> SMKLDIKKTFSNRSDRVKGIDFHPTEPWVLTTLYSGRVEIWNYETQVEVRSIQVTETPVRAGKFIARKNWIIVGSDDFRIRVFNYNTGEKVVDFEAHPDYIRSIAVHPTKPYVLSGSDDLTVKLWNWENNWALEQTFEGHEHFVMCVAFNPKDPSTFASGCLDRTVKVWSLGQSTPNFTLTTGQERGVNYVDYYPLPDKPYMITASDDLTIKIWDYQTKSCVATLEGHMSNVSFAVFHPTLPIIISGSEDGTLKIWNSSTYKVEKTLNVGLERSWCIATHPTGRKNYIASGFDNGFTVLSLG;> GVKLHYT

Hence, this loss of critical proteins has the potential to compromise ER proteostasis and generate cellular stress. This challenge to normal metabolism is overcome by the activity of the cytosolic coatomer protein I (COPI) polymer, whose repeating unit is the coatomer, a 560 kDa complex of seven distinct gene products (α-, β-, β′-, γ-, δ-, ε-, and ζ-COPI)25–31. Overall, the coatomer functions to retrieve the escaped “client” proteins, such as type I membrane proteins, from cis-Golgi back to ER by retrograde trafficking. In particular, the S protein – a type I membrane protein – is delivered to the ERGIC from both the ER (by anterograde trafficking) and the Golgi (by retrograde trafficking)3,10–12. Here we utilize recombinant SARS-CoV-2 S proteins and tail peptides, including constructs with enhanced mimicry of the coatomer binding motif (clientized S protein), to elucidate the atomic structure of the S-coatomer interface.

To determine an atomic-level understanding of S-coatomer interactions, we attempted co-crystallization of αWD40 with either wild-type (1267Gly-Val-Lys-Leu-His-Tyr-Thr1273) or clientized (1267Gly-Val-Lys-Leu-His-Tyr-Glu1273) S tail heptapeptides. However, in our co-crystallization experiments, contacts between symmetry-related αWD40 molecules occluded the binding site and no S tail peptide density was observed. Hence, we subsequently adopted a previously described strategy of using β‘WD40 for co-crystallization of peptides containing the Lys-x-His-x-xCT motif 61, which was also used for structural investigations of S tail peptides, recently during the revision of this manuscript. The β‘WD40 co-crystal structures with the wild-type and clientized Thr127Glu S heptapeptides were determined to a resolution of 1.4 Å. Overall, these two crystal structures reveal substantial similarity (Cα RMSD = 0.2 Å). The S tail heptapeptides are intercalated between two stacked β‘WD40 domains. The S tail extended motif makes contact with the binding site residues in one of the two β‘WD40 domains whereas the upstream tail residues interact with the other β‘WD40 domain, but at the face distal from the binding site. The major difference is that whereas only the main chain carboxylate of wild-type Thr1273 interacts with basic Lys17 on the β‘WD40 surface, both the side chain and main chain carboxylate groups of the clientized Glu1273 residue form extensive interactions with a β’WD40 basic cluster of Arg15, Lys17, and Arg272. A Thr1273 in wild-type S shows no side-chain interactions with the basic cluster. Overall, the two heptapeptides occupy the canonical WD40 binding site, which provides electrostatic complementarity to the dibasic motif residues, Lys1269 and His1271. C The β‘WD40 surface provides electrostatic complementarity to the S dibasic motif and the C-terminus.Building on the previously established methods in assembling enterovirus RdRP EC and in capturing various EC states, we used an EV71 RdRP bearing a C291M mutation in such approaches, since the equivalent PV RdRP mutant (C290M) was shown to produce higher quality EC crystals. Building on our recent work reporting an enterovirus 71 (EV71) RdRP EC with an intermediate conformation of its template-product duplex, here we report three types of translocation intermediate crystal structures that define multiple nucleic acid conformations bridging the pre- and post-translocation states, both in the regulate forward translocation and in an unusual reverse translocation induced by pyrophosphate (PPi) and divalent metal ions. These structural data, in combination with enzymology characterization of the RdRP, highlight the key role of RdRP motif G in controlling the critical movement of the template RNA strand that is probably the rate-limiting step for both forward and reverse translocations. A striking common feature for both modes of translocation is that the template backbone, in particular for positions −2 to +1, stayed fixed relative to its starting point of translocation. As we pointed out previously, this phenomenon is probably related to two motif G residues (T114-S115 in EV71 RdRP, “G” symbol in Figs. 2d and 3d) that create a hurdle-like steric blockage right at the +1/+2 junction of the template backbone.

While the template strand density of this type of structure appeared normal, the density of the product strand clearly indicated the presence of two sets of backbone phosphates. When a pre-translocation product RNA was modeled, strong positive density appeared between the modeled phosphates and continuous density was observed for an array of neighboring product bases. By modeling two alternate conformations of the product strand, this unusual density can be readily interpreted. Accordingly to the six-state nomenclature of the RdRP NAC suggested in our previous work with S6 representing translocation intermediates, we assign these two EC states as S6A and S6B. While both states share the same template model that is nearly identical to that in the previously reported S6 structure, the two product models differ in the extent of translocation with S6B leading S6A with an occupancy of 60% and 40%, respectively. Comparing to the S5 product RNA, the S6A product slightly moved toward the upstream as an entity, while the S6B product had the upstream nucleotides move by longer distances than the downstream nucleotides and is nearly identical to the previously reported S6 product (Supplementary Movie 1: the first clip shows the modeled transition from S5 to S6).

> GEIQWVKPNKETGRLNINGPTRTKLEPSVFHDVFEGNKEPAVLHSKDPRLEVDFEQALFSKYVGNTLYEPDEYIKEAALHYANQLKQLDIDTSQMSMEEACYGTENLEAIDLHTSAGYPYSALGIKKRDILDSTTRDVSKMKFYMDKYGLDLPYSTYVKDELRSIDKIKKGKSRLIEASSLNDSVYLRMTFGHLYETFHANPGTVTGSAVGCNPDTFWSKLPILLPGSLFAFDYSGYDASLSPVWFRALELVLREIGYSEEAVSLVEGINHTHHVYRNKTYCVLGGMPSGMSGTSIFNSMINNIIIRALLIKTFKGIDLDELNMVAYGDDVLASYPFPIDCLELARTGKEYGLTMTPADKSPCFNEVNWDNATFLKRGFLPDEQFPFLIHPTMPMKEIHESIRWTKDARNTQDHVRSLCLLAWHNGKQEYEKFVSAIRSVPVGKALAIPNYENLRRNWLELFHHHHHH> VDLGTENLYFQSADTLPVAAAFTETVNAYFKGADPSKCIVKITGEMVLSFPAGITRHFANNPSPAALTFRVINFSRLEHVLPNPQLLCCDNTQNDANTKEFWVNMPNLMTHLKKVSEQKPQATYYNVDMLKYQVSAQGIQSTPLNLAVNWRCEPSSTDLRIDYKYNTDAMTTAVALNNVQFLVPIDGGVTKLQAVLPPAVWNAEQQRILWKIPDIS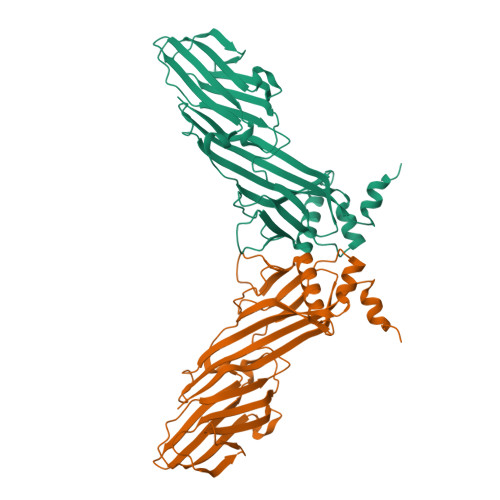QKSENGGVGSLLARFQLSEGPSKPSPLVVQFTSEGSTLSGCDIELVGAGYRFSLIKKRFAAGKYLADN> MADSDINIKTGTTDIGSNTTVKTGDLVTYDKENGMHKKVFYSFIDDKNHNKKLLVIRTKGTIAGQYRVYSEEGAN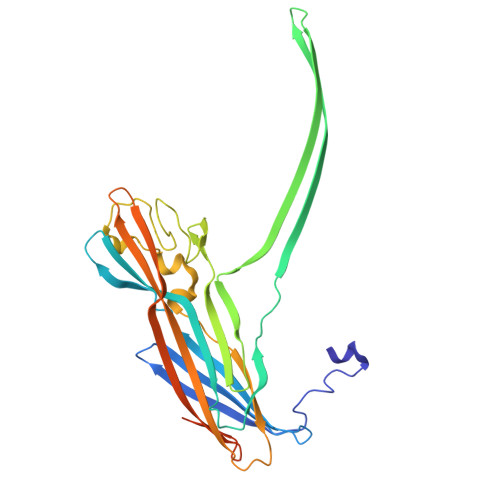KSGLAWPSAFKVQLQLPDNEVAQISDYYPRNSIDTKEYMSTLTYGFNSNVTGDDTGKIGGLIGANVSIGHTLRYVQPDFKTILESPTDKKVGWKVIFNNMVNQNWGPYDRDSWNPVYGNQLFMKTRNGSMKAADNFLDPNKASSLLSSGFSPDFATVITMDRCASKQQTNIDVIYERVRDDYQLHWTSTNWKGTNTKDKWTDRSSERYKIDWEKEEMTNGSSGSRGVPHIVMVDAYKRYKGGSHHHHHH> FQKIYSPTQLANAMKLVRQQNGWTQSELAKKIGIKQATISNFENNPDNTTL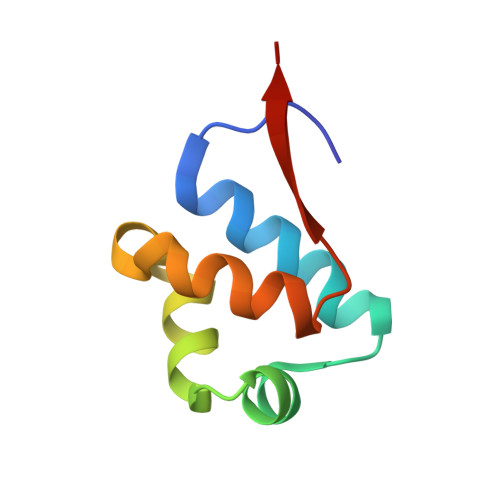TTFFKILQSLELSMTLCDAK> GSHMKNSVSVDLPGSMKVLVSKSSNADGKYDLIATVDALELSGTSDKNNGSGVLEGVKADASKVKLTISDDLGQTTLEVFKSDGSTLVSKKVTSKDKVLGDVKFNEKGEVSEKIITRADGTRLEYTGIKSDGSGKAKEVLKGYVLEGTLTAEKT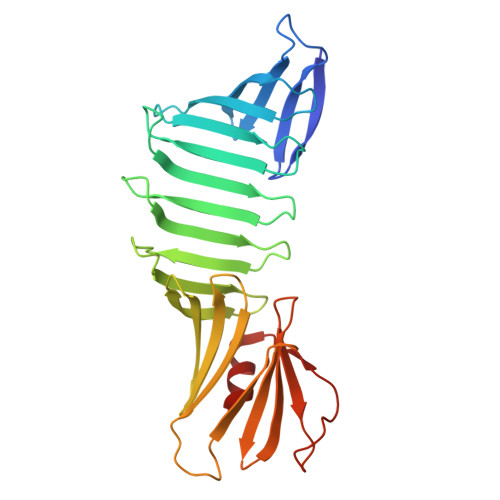TLVVKEGTVTLSKNISKSGAVSVELNDTDSSAATKKTAAWNSGTSTLTITVNSKKTKDLVFTSSNTITVQQYDSNGTSLEGSAVEITKLDEIKNALK>[4x]PDA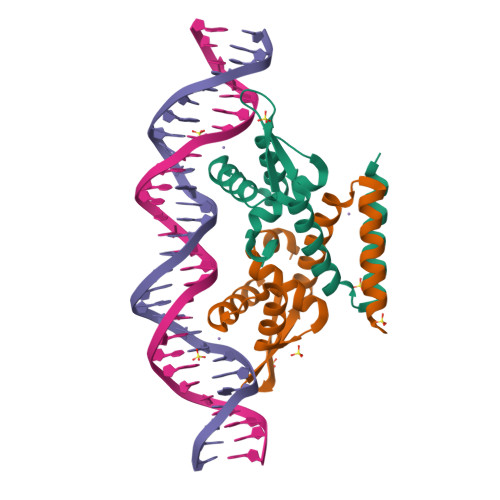RSDARDLTAFQKNILTVLGEEARYGLAIKRELEEYYGEEVNHGRLYPNLDDLVNKGLVEKSELDKRTNEYALTNEGFDAVVDDLEWTLSKFVADADRRERVETIVADDAAALEH>[2x]CPRFLKVKNWETDVVLTDTLHLKSTLETGCTEHICMGSIMLPSQHTRKPEDVRTKDQLFP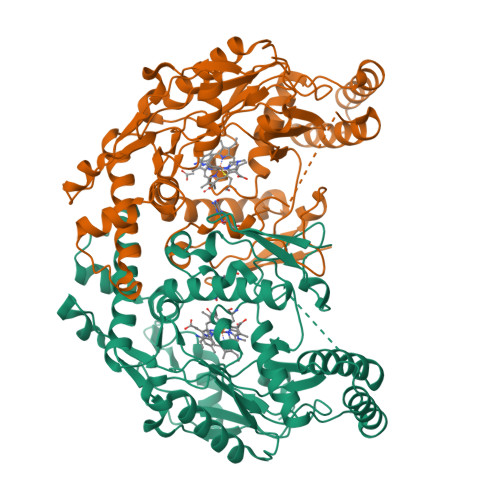LAKEFLDQYYSSIKRFGSKAHMDRLEEVNKEIESTSTYQLKDTELIYGAKHAWRNASRCVGRIQWSKLQVFDARDCTTAHGMFNYICNHVKYATNKGNLRSAITIFPQRTDGKHDFRVWNSQLIRYAGYKQPDGSTLGDPANVQFTEICIQQGWKAPRGRFDVLPLLLQANGNDPELFQIPPELVLEVPIRHPKFDWFKDLGLKWYGLPAVSNMLLEIGGLEFSACPFSGWYMGTEIGVRNYCDNSRYNILEEVAKKMDLDMRKTSSLWKDQALVEINIAVLYSFQSDKVTIVDHHSATESFIKHMENEYRCRGGCPADWVWIVPPMSGSITPVFHQEMLNYRLTPSFEYQPDPWNTHVWKG>[2x]PSVYDAAAQLTADVKKDLRDSWKVIGSDKKGNGVALMTTLFADNQETIGYFKRLGDVSQGMANDKLRGHSIGLMYALQNFIDQLDNPDDLVCVVEKFAVNH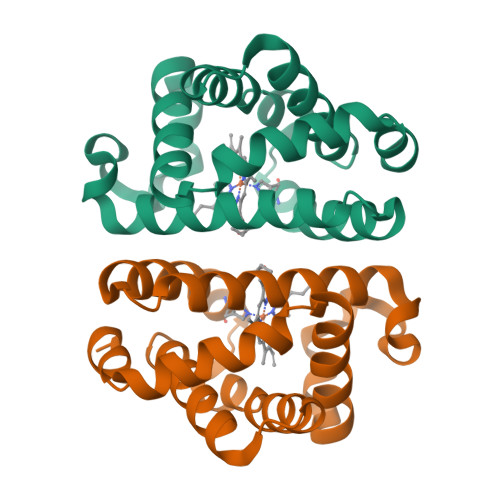ITRKISAAEFGKINGPIKKVLASKNFGDKYANAWAKLVAVVQAAL>[2x]MTKFSGNELRAELYRRAFLSYSVAPGALGMFGRSLLAKGARAEALANGTVMSGSHWGVFTATVENGRATAFTPWEKDPHPS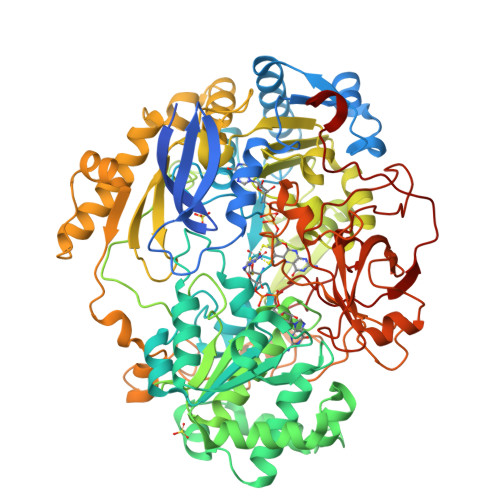PMLAGVLDSIYSPTRIKYPMVRREFLEKGVNADRSTRGNGDFVRVSWDQALDLVAAEVKRVEETYGPEGVFGGSYGWKSPGRLHNCTTLLRRMLTLAGGYVNGAGDYSTGAAQVIMPHVVGTLEVYEQQTAWPVLAENTEVMVFWAADPIKTSQIGWVIPEHGAYPGLEALKAKGTKVIVIDPVRTKTVEFFGAEHITPKPQTDVAIMLGMAHTLVAEDLYDKDFIANYTSGFDKFLPYLDGETDSTPKTAEWAEGISGVPAETIKELARLFESKRTMLAAGWSMQRMHHGEQAHWMLVTLASMLGQIGLPGGGFGLSYHYSGGGTPSTSGPALAGITDGGAATKGPEWLAASGASVIPVARVVDMLENPGAEFDFNGTRSKFPDVKMAYWVGGNPFVHHQDRNRMVKAWEKLETFVVHDFQWTPTARHADIVLPATTSYERNDIETIGDYSNTGILAMKKIVEPLYEARSDYDIFAAVAERLGKGAEFTEGKDEMGWIKSFYDDAAKQGKAAGVEMPAFDAFWAEGIVEFPVTDGADFVRYASFREDPLLNPLGTPTGLIEIYSKNIEKMGYDDCPAHPTWMEPLERLDGPGAKYPLHIAASHPFNRLHSQLNGTVLREGYAVQGHEPCLMHPDDAAARGIADGDVVRVHNDRGQILTGVKVTDAVMKGVIQIYEGGWYDPSDVTEPGTLDKYGDVNVLSADIGTSKLAQGNCGQTVLAEVEKYTGPAVTLTGFVAPKAAE>[2x]MLGLKTSIIGRRVIYFQEITSTNEFAKTSYLEEGTVIVADKQTMGHGRLNRKWESPEGGLWLSIVLSPKVPQKDLPKIVFLGAVGVVETL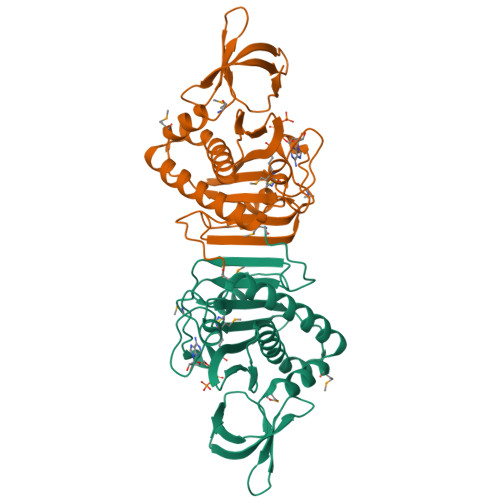KEFSIDGRIKWPNDVLVNYKKIAGVLVEGKGDKIVLGIGLNVNNKVPNGATSMKLELGSEVPLLSVFRSLITNLDRLYLNFLKNPMDILNLVRDNMILGVRVKILGDGSFEGIAEDIDDFGRLIIRLDSGEVKKVIYGDVSLRFL>MAKRIQFSATGGPEVLEYVDFEPKDPAAGEVQVENKAIGINYIDTYVRSGLYPAPLPSGLGSEAAGVVTKVGTGVSHIKVGDRVVYAQSSLGAYSEYHNVPAQKVAVLPEGISFEQAAASFLKGLTVQYLFRQ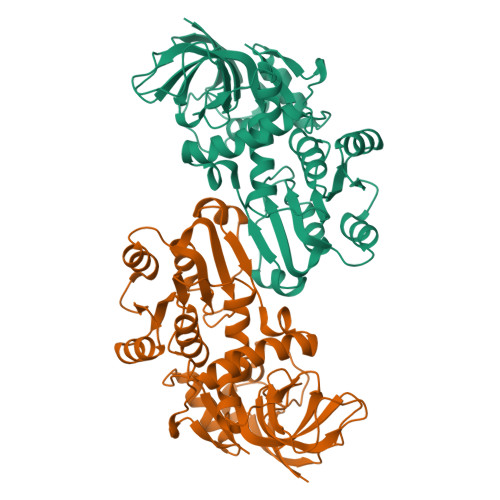THKIKAGDIFLFHAAAGGVGLIASQWAKALGAKLIGTVGSDEKAALAKEAGAWATINYQTEDIAARVAELTQGEKVSVVYDSVGKSTWLASLDSLKRHGLLVSFGNASGPVKDVDLGILNQKGSLFVTRPSLNGYITTQEELAAASEELFSLIASDAIKVDVKDAQKFPLSQARRAHETLESRATTGSSLLIP[2x]> LKAGPLLSSEKLIAIGASTGGTEAIRHVLQPLPLSSPAVIITQHMPPGFTRSFAERLNKLCQISVKEAEDGERVLPGHAYIAPGDKHMELARSGANYQIKIHDGPPVNRHRPSVDVLFHSVAKHAGRNAVGVILTGMGNDGAAGMLAM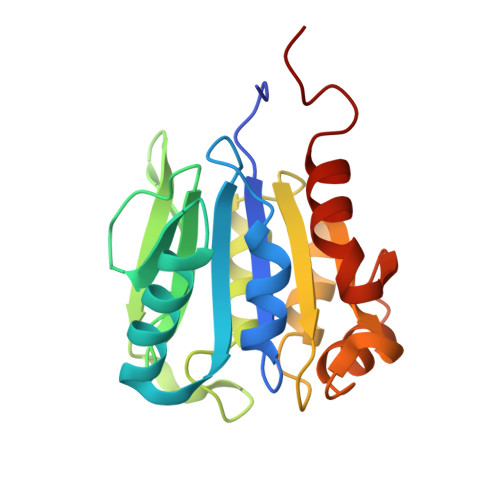YQAGAWTIAQNEASCVVFGMPREAINMGGVSEVVDLSQVSQQMLAKISAGQAIRI>[6x]EFMLELAILGLLIESPMHGYELRKRLTGLLGAFRAFSYGSLYPALRRMQADGLIAENAAPAGT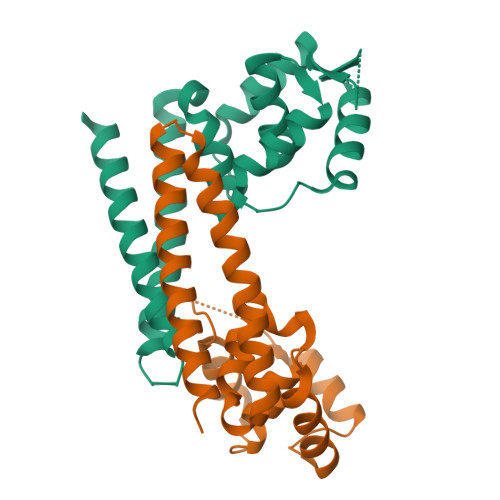PVRRARRVYQLTDKGRRRFGELVADTGPHNYTDDGFGVHLAFFNRTPAEARMRILEGRRRQVEERREGLREAVARASSSFDRYTRQLHQLGLESSEREVKWLNELIAAERAAPNPAEQT4-({(4S,5R)-4,5-bis(4-chlorophenyl)-2-[4-methoxy-2-(propan-2-yloxy)phenyl]-4,5-dihydro-1H-imidazol-1-yl}carbonyl)piperazin-2-one | C30 H30 Cl2 N4 O4 | 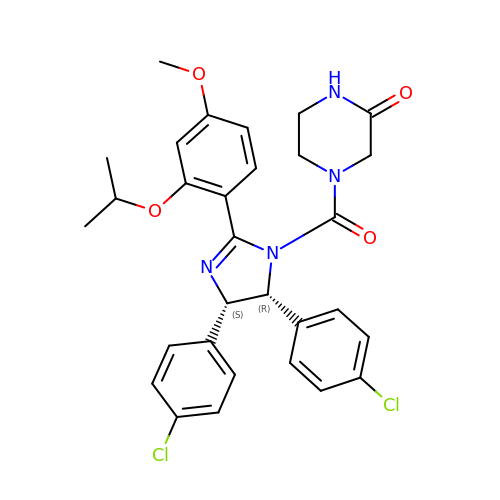BDUHCSBCVGXTJM-WUFINQPMSA-N> MGHHHHHHSHMSGEKTVVCKHWLRGLCKKGDQ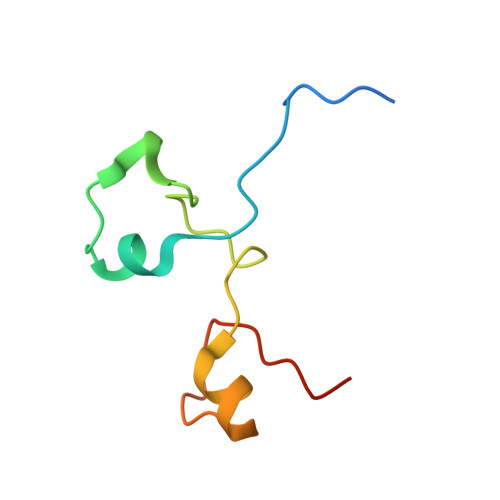CEFLHEYDMTKMSECYFYSKFGECSNKECPFLHIDPESKI>MDATALERDAVQFARLAVQRDHEGRYSEAVFYYKEAAQALIYAEMAGSSLENIQEKITEYLERVQALHSAVQSKSADPLKSKHQLDLERAHFLVTQAFDEDEKENVEDAIELYTEAVDLCLKTSYETADKVLQNKLKQLARQALDRAEALSEPLTKPVGKISSTS[2x];>NFVLPELPSVPDTLPTASAGASTSASEDIDFDDLSRRFEELKKKT[2x]

One such cofactor was Calpain-7 (CAPN7), a ubiquitously expressed but poorly understood cysteine protease that had not previously been linked to abscission or to the NoCut checkpoint. CAPN7 contains tandem MIT domains that can bind specifically to the ESCRT-III subunit IST1. Many of these cofactors contain microtubule-interacting and trafficking (MIT) domains, which bind differentially to MIT-interacting motifs (MIMs) located near the C termini of the different human ESCRT-III proteins. Hence, IST1 recruits CAPN7 to midbodies, where its proteolytic activity is required to regulate and complete abscission.

We determined the crystal structure of the CAPN7(MIT)2–IST1322-366 complex to define the interaction in molecular detail and distinguish between the four possible binding modes in which individual CAPN7 MIT domains either bound simultaneously to both IST1 MIMs, as reported in other MIT:MIM interactions, or each CAPN7 MIT domain bound a different IST1 MIM element in one of two possible pairwise interactions. The structure revealed that each MIT domain binds a different MIM element, which is a configuration that has not been documented previously. The asymmetric unit contains two copies of the CAPN7(MIT)2 –IST1322-366 complex, and the flexible linkers between the different MIT and MIM elements could, in principle, connect the linked IST1 MIM-CAPN7 complexes in two different ways. The N-terminal IST1 MIM element binds in an extended conformation in the helix 1/3 groove of the N-terminal CAPN7 MIT domain, making a canonical ‘type 2’ (MIM2) interaction (Kieffer et al., 2008; Samson et al., 2008; Vild and Xu, 2014; Kojima et al., 2016; Wenzel et al., 2022). The binding interface spans IST1 residues 324–332 (324VLPELPSVP332), which resembles the previously defined MIM2 consensus sequence (ΦPXΦPXXPΦP, where Φ represents a hydrophobic residue and X a variable (often polar) residue; Kojima et al., 2016). In the CAPN7-IST1 complex, IST1 Ser330 bulges away from the MIT domain to accommodate an intramolecular salt bridge formed by CAPN7 Asp21 and Arg63, and the peptide then bends back to allow Val331 and Pro332 to make hydrogen bonds and hydrophobic contacts, respectively. The C-terminal IST1 MIM element (349DIDFDDLSRRFEELKK364) forms an amphipathic helix that packs between helices 1 and 3 of the C-terminal CAPN7 MIT domain, making a canonical ‘type 3’ (MIM3) interaction (Yang et al., 2008; Skalicky et al., 2012; Wenzel et al., 2022). Core residues from the hydrophobic face of the IST1 helix are buried in the CAPN7 MIT helix 1/3 groove, and the interface hydrophobic contacts, hydrogen bonds, and salt bridges are nearly identical to those seen when this same IST1 motif makes a type 3 interaction with the MIT domain of SPARTIN (Guo and Xu, 2015; Wenzel et al., 2022).> GSHMASPNGQTKPLPALKLALEYIVPAMNKHGICVVDDFLGKETGQQIGDEVRALHDTGKFTDGQLVSQKSDSSKDIRGDKITWIEGKEPGCETIGLLMSSMDDLIRHCNGKLGSYKINGRTKAMVACYPGNGTGYVRHVDNPNGDGRCVTCIYYLNKDWDAKVSGGILRIFPEGKAQ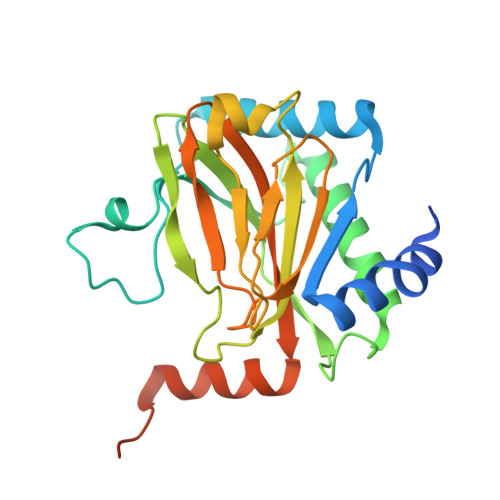FADIEPKFDRLLFFWSDRRNPHEVQPAYATRYAITVWYFDADERAAAKVKYLTGEKGVRVELNKPSDSVGKDVF> QSSSASPQEQDQDRRKDWGHVELLEVLQARVRQLQAESVSEVVVNRVDVARLPECGSGDGSLQPPRKVQMGAKDATPVPCGRWAKILEKDKRTQQMRMQRLKAKLQMPFQSGEFKALTRRLQVEPRLLSKQMAGCLEDCTRQAPESPWEEQLARLLQEAPGKLSLDVEQAPSGQHSQAQLSGQQQRLLAFFKCCLLTDQLPLAHHLLVVHHGQAQKRALLTLDMYNAVMLGWARQGAFKELVYVLFMVKDAGLTPDLLSYAAALQCMGRQDQDAGTIERCLEQMSQEGLKLQALFTAVLLSEEDRATVLKAVHKVKPTFSLPPQLPPPVNTSKLLRDVYAKDGRVSYPKLHLPLKTLQCLFEKQLHMELASRVCVVSVEKPTLPSKEVKHARATLATLRDQWEKALCRALRETKNRLEREVYEGRFSLYPFLCLLDEREVVRMLLQVLQ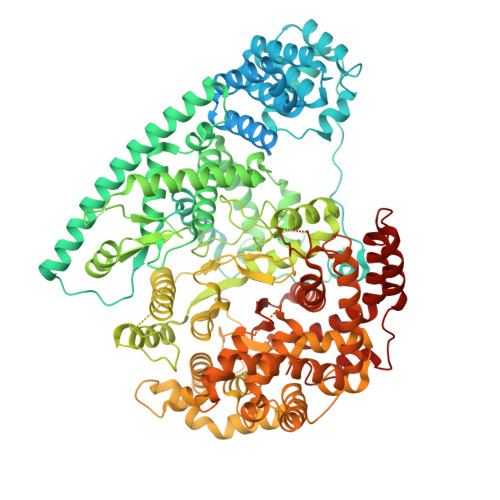ALPAQGESFTTLARELSARTFSRHVVQRQRVSGQVQALQNHYRKYLCLLASDAEVPEPCLPRQYWEELGAPEALREQPWPLPVQMELGKLLAEMLVQATQMPCSLDKPHRSSRLVPVLYHVYSFRNVQQIGILKPHPAYVQLLEKAAEPTLTFEAVDVPMLCPPLPWTSPHSGAFLLSPTKLMRTVEGATQHQELLETCPPTALHGALDALTQLGNCAWRVNGRVLDLVLQLFQAKGCPQLGVPAPPSEAPQPPEAHLPHSAAPARKAELRRELAHCQKVAREMHSLRAEALYRLSLAQHLRDRVFWLPHNMDFRGRTYPCPPHFNHLGSDVARALLEFAQGRPLGPHGLDWLKIHLVNLTGLKKREPLRKRLAFAEEVMDDILDSADQPLTGRKWWMGAEEPWQTLACCMEVANAVRASDPAAYVSHLPVHQDGSCNGLQHYAALGRDSVGAASVNLEPSDVPQDVYSGVAAQVEVFRRQDAQRGMRVAQVLEGFITRKVVKQTVMTVVYGVTRYGGRLQIEKRLRELSDFPQEFVWEASHYLVAQVFASLQEMFSGTRAIQHWLTESARLISHMGSVVEWVTPLGVPVIQPYRLDSKVKQIGGGIQSITYTHNGDISRAPNTAKQANGFPPNFIHSLDSSHMMLTALHCYRKGLTFVSVHDCYWTHAADVSVMNQVCREQFVRLHSEPILQDLSRFLVKRFCSEPQKILEASQLKETLQAVPKPGAFDLEQVKRSTYFFS>SMKAASIIERLAAGQVHVYPRSRHESEGTRVQMIKAEGRKYLVAEGSGKLYDELRGEEADGVKLCELSHENRLVLNRHFPFTVPQAFGKQSATIGLGDRLGIAGPGHVQTVRGRAIHPILAQQSIRELALTGRDYKQVIDAAAYAVFQEGYTEGYGADGDHLKKEEDIRMALDLGFTMLTLDCSEQIDNEAAQAGESEVKRKYEELPESVRSHYEAKYLDKTFQVGPHAIHFDAATLMRDVLVYREAIQFMIYIYEKYIQTAGRAVDFEISIDETLAPTAPGSHFLVASELIGKNVDIFSMAPRFIGEFQKGIDYIGDIAQFERELAVHAAIADRFGYKLSIHSGSDKFSVFALVGRYTNGRFHVKTAGTNWLEAVRIVAKTNPGLYRRMH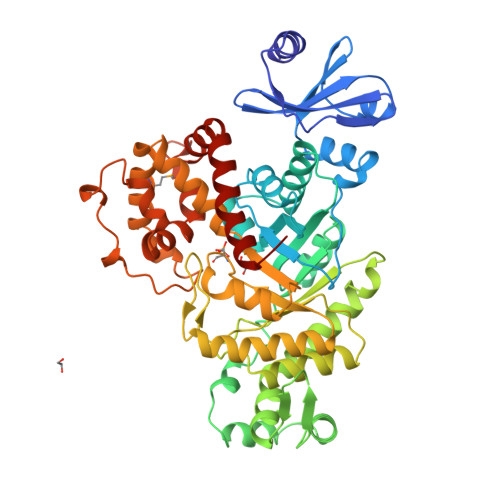QYALEHFEEATAYYHVTTNLNNIRPLADVSDEELPSYMNENDARQLLHITYGLLLQAKKDDGSSLFRDEFFRTLSEREEDYEAALRSHIGKHLDLLGVK[2x]>[2x]GSGMRFYVKDHRNKAMINLHIQ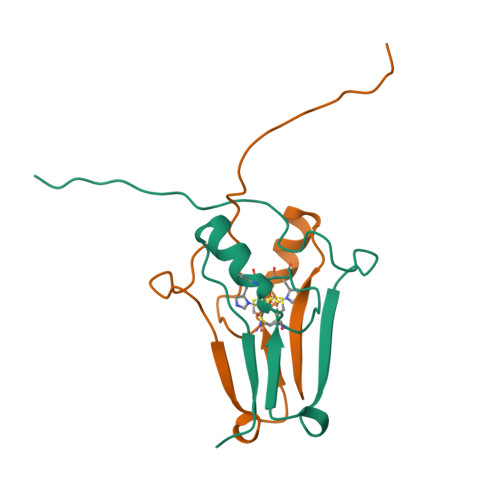KDNPKIVHAFDMEDLGDKAVYCRCWRSKKFPFCDGAHTKHNEETGDNVGPLIIKKKET>[2x]GSSGSSGQTELNDFLLDVSKTYFDNIVAIDSLLEHIMIYAKNLVNADRCALFQVDHKNKELYS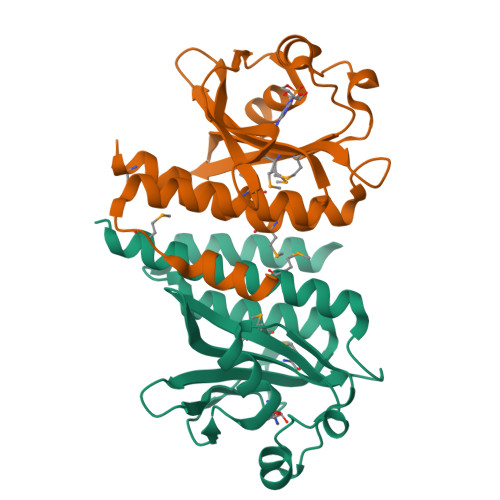DLFDIGEEKEGKPVFKKTKEIRFSIEKGIAGQVARTGEVLNIPDAYADPRFNREVDLYTGYTTRNILCMPIVSRGSVIGVVQMVNKISGSAFSKTDENNFKMFAVFCALALHCANMYHRIRHSECI A number of enzymes, termed fructosyl amino acid oxidase (FAOX), have reactivity for fructosyl amino acids as major substrates. Some of these enzymes, which also exhibit reactivity for fructosyl dipeptides as F-VH are specifically termed fructosyl peptide oxidase (FPOX). AnFPOX-15, which featured 11 amino acid replacements in AnFPOX-1 exhibited significant F-VH oxidation activity, whereas reactivity for longer fructosyl peptides such as fructosyl tripeptide (F-3P, Fru-VHL), fructosyl tetrapeptide (F-4P, Fru-VHLT) and F-6P was never observed. The overall structure of AnFPOX-15 consisted of two domains: an oxidoreductase FAD-binding domain with the topology of an incomplete anti-parallel β-barrel (two β-sheets with eight β-strands) and four α-helices at one side of the β-barrel; and a catalytic domain with two β-sheets (eight or two β-strands), and two long α-helices (helix 2 and 3) that locate at each side of the sheets, and some short helices.

The first-generation mutants, in which R61 was replaced with glycine or alanine, displayed significant oxidation activities for F-6P. To confirm the structural influence of the R61G mutation, the crystal structure of AnFPOX-15 R61G was determined. Ligand-free AnFPOX-15 R61G and AnFPOX-15 R61G/FSA structures were crystallised under similar condition as those used for AnFPOX-15, and the structures were determined via molecular replacement using coordinates of AnFPOX-15 as the initial model. No other significant structural differences were found between AnFPOX-15 and AnFPOX-15 R61G (rmsd = 0.148 Å for 431 Cα atoms). As well as in the case of AnFPOX-15, no significant structural difference was observed between the ligand-free AnFPOX-15 R61G and AnFPOX-15 R61G/FSA (rmsd = 0.17 Å for 431 Cα atoms). From these observations, the generated R61G mutant acquired significant oxidation activity for F-6P, and the wider space of substrate gate in R61G mutant was confirmed via its crystal structure.

> MAPRANTKIIVVGGGGTMGSSTALHLLRAGYTPSNITVLDTYPIPSAQSAGYDLNKIFGIGLRNKPDLQLYLEALDMWKNDPLFKPFFHNVGQMDVSSTEEGIKKLRMRYQSLLDAGIGLEKTNFLLESEDEILAKAPHFTREQIKGWKGLFCGDGGWLAAAKAINAIGQFLKEQGVKFGFGEAGTFKKPLFADADEKTCIGVETVDGTKYYADKVVLAAGAWSSTLVDLEEQCVSKAWVFAHIQLTPAEAAAYKNTPVIYDGDYGFFIEPDENGIIKVCDEFPGFTHFKMHQPYGSPVPKLISVPRSHAKHPTDTYPHASEVTIKKAINRFLPRFNDKELFNRAMCWCTDTADANLLVCEHPRWKGFYLATGDSGHSFKLLPNIGKHVVELLEGRLESVFKDAWRWRPGSGDALKSRRAAPAKDLADMPGWRNEAKM> AAPTAYTPLDVAQAYQFPEGLDGQGQCIAIIELGGGYDEASLAQYFASLGVPAPQVVSVSVDGASNQPTGDPSGPDGHVELDIEVAGALAPGAKFAVYFAPNTDAGFLDAITTAIHDPTLKPSVVSISWGGPEDSWTSAAIAAMNRAFLDAAALGVTVLAAAGDSGSTDGEQDGLYHVDFPAASPYVLACGGTRLVASGGRIAQETVWNDGPDGGATGGGVSRIFPLPAWQEHANVPPSANPGASSGRGVPDLAGNADPATGYE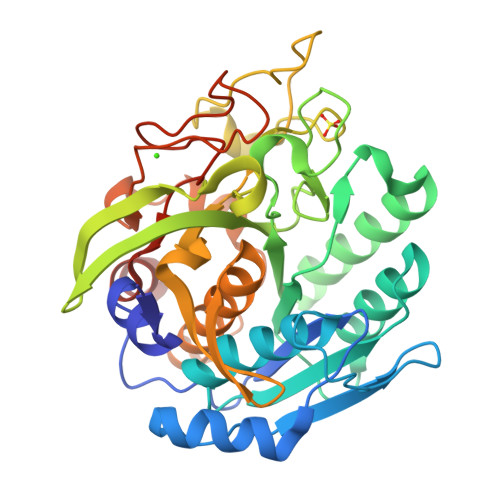VVIDGEATVIGGTSAVAPLFAALVARINQKLGKAVGYLNPTLYQLPADVFHDITEGNNDIANRAQIYQAGPGWDPCTGLGSPIGVRLLQALLPSASQPQP> MVTQTNPVPVTYPTDAYIPTYLPDDKVSNLADLKKLIEMDSRLDLYLTRRRLDTSINLPTNTKTKDHPPNKEMLRIYVYNTTES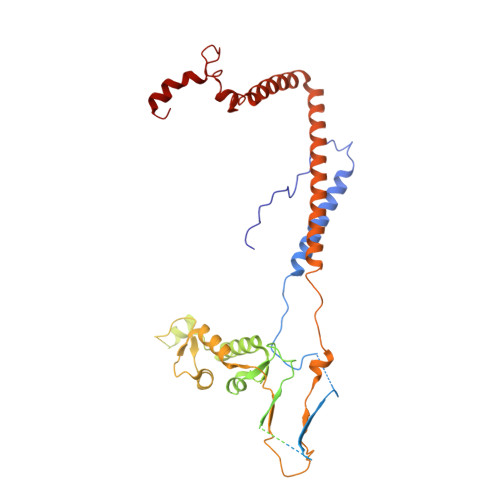SPRSDSGTPADSGKTTWTLRIEGKLLHESANGKHPFSEFLEGVAVDFKRLKPLGMGKKRKRDSSLSLPLNLQQPEYNDQDSTMGDNDNGEDEDSAEAESREEIVDALEWNYDENNVVEFDGIDIKRQGKDNLRCSITIQLRGVDGGKVQYSPNLATLIGMQTGSVNDAVYSIYKYILINNLFVTEQTEAQDGSNDAEDSSNENNNKNGAGDDDGVEGSTPKDKPELGEVKLDSLLQKVLDTNAAHLPLMNVVQTVNKLVSPLPPIILDYTIDLSKDTTYGATTLDVDVSHILHQPQPQPNLQKEEETDAEDTAKLREITKLALQLNSSAQKYQFFHELSLHPRETLTHYLWSSKQNELVLQGDQYFNEDAARTSDIYSNNNNDRSLMGNISLLYSQGRL>[4x]MLSRKGIIPEEYVLTRLAEDPTEPRYRTRERRARFVSKKGNCNVAHKNIREQGRFLQDVFTTLVDLKWPHTLLIFTMSFLCSWLLFAMVWWLIAFAHGDLAPGEGTNVPCVTSIHSFSSAFLFSIEVQVTIGFGGRMVTEECPLAILILIVQNIVGLMINAIMLGCIFMKTAQAHRRAETLIFSKHAVITPRHGRLCFMLRVGDLRKSMIISATIHMQVVRKTTSPEGEVVPLHQVDIPMENGVGGNSIFLVAPLIIYHVIDSNSPLYDLAPSDLHHHQDLEIIVILEGVVETTGITTQARTSYLADEILWGQRFVPIVAEEDGRYSVDYSKFGNTVKVPTPLCTARQLDEDRSLLDALTLASSRGPLRKRSVAVAKAKPKFSISPDSLS;>DYKDDDDKMPLAFCGTENHSAAYRVDQGVLNNGCFVDALNVVPHVFLLFITFPILFIGWGSQSSKVHIHHSTWLHFPGHNLRWILTFILLFVLVCEIAEGILSDGVTESRHLHLYMPAGMAFMAAITSVVYYHNIETSNFPKLLIALLIYWTLAFITK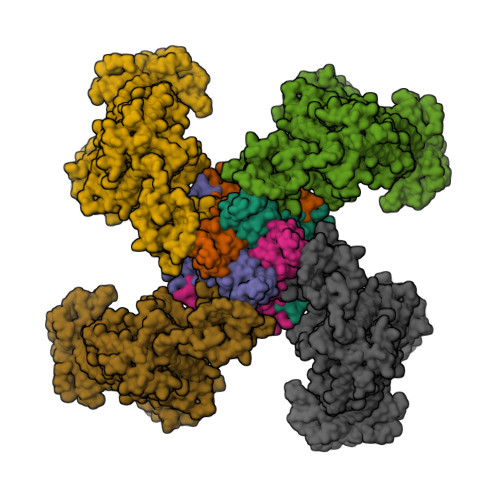TIKFVKFYDHAIGFSQLRFCLTGLLVILYGMLLLVEVNVIRVRRYIFFKTPREVKPPEDLQDLGVRFLQPFVNLLSKGTYWWMNAFIKTAHKKPIDLRAIAKLPIAMRALTNYQRLCVAFDAQARKDTQSPQGARAIWRALCHAFGRRLILSSTFRILADLLGFAGPLCIFGIVDHLGKENHVFQPKTQFLGVYFVSSQEFLGNAYVLAVLLFLALLLQRTFLQASYYVAIETGINLRGAIQTKIYNKIMHMSTSNLSMGEMTAGQICNLVAIDTNQLMWFFFLCPNLWTMPVQIIVGVILLYYILGVSALIGAAVIILLAPVQYFVATKLSQAQRTTLEHSNERLKQTNEMLRGMKLLKLYAWESIFCSRVEVTRRKEMTSLRAFAVYTSISIFMNTAIPIAAVLITFVGHVSFFKESDLSPSVAFASLSLFHILVTPLFLLSSVVRSTVKALVSVQKLSEFLSSAEIREEQCAPREPAPQGQAGKYQAVPLKVVNRKRPAREEVRDLLGPLQRLAPSMDGDADNFCVQIIGGFFTWTPDGIPTLSNITIRIPRGQLTMIVGQVGCGKSSLLLATLGEMQKVSGAVFWNSNLPDSEGEDPSSPERETAAGSDIRSRGPVAYASQKPWLLNATVEENITFESPFNKQRYKMVIEACSLQPDIDILPHGDQTQIGERGINLSGGQRQRISVARALYQQTNVVFLDDPFSALDVHLSDHLMQAGILELLRDDKRTVVLVTHKLQYLPHADWIIAMKDGTIQREGTLKDFQRSECQLFEHWKTLMNRQDQELEKETVMERKASEPSQGLPRAMSSRDGLLLDEEEEEEEAAESEEDDNLSSVLHQRAKIPWRACTKYLSSAGILLLSLLVFSQLLKHMVLVAIDYWLAKWTDSALVLSPAARNCSLSQECDLDQSVYAMVFTLLCSLGIVLCLVTSVTVEWTGLKVAKRLHRSLLNRIILAPMRFFETTPLGSILNRFSSDCNTIDQHIPSTLECLSRSTLLCVSALTVISYVTPVFLVALLPLAVVCYFIQKYFRVASRDLQQLDDTTQLPLVSHFAETVEGLTTIRAFRYEARFQQKLLEYTDSNNIASLFLTAANRWLEVCMEYIGACVVLIAAATSISNSLHRELSAGLVGLGLTYALMVSNYLNWMVRNLADMEIQLGAVKRIHALLKTEAESYEGLLAPSLIPKNWPDQGKIQIQNLSVRYDSSLKPVLKHVNTLISPGQKIGICGRTGSGKSSFSLAFFRMVDMFEGRIIIDGIDIAKLPLHTLRSRLSIILQDPVLFSGTIRFNLDPEKKCSDSTLWEALEIAQLKLVVKALPGGLDAIITEGGENFSQGQRQLFCLARAFVRKTSIFIMDEATASIDMATENILQKVVMTAFADRTVVTIAHRVHTILSADLVMVLKRGAILEFDKPETLLSQKDSVFASFVRADK[4x]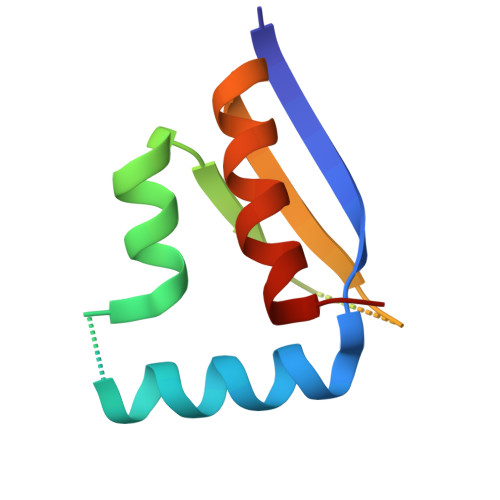>[4x]SMSEERFRVDRKKLEAMLQAAAEGKGRSGEDFFQKIMEETNTQIAWPSKLKIGAKSKKDPHIKVSGKKEDVKEAKEMIMSVLDTKS> MAHHHHHHVGTDDWRCARSMHEFSAKDIDGHMVNLDKYRGFVCIVTNVASQCGKTEVNYTQL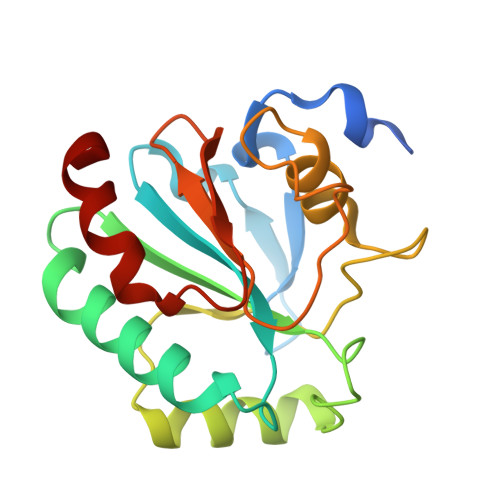VDLHARYAECGLRILLFPCNQFGKQEPGSNEEIKEFLAGYNFKGDAFSKICVNGDDAHPLWKWMKIQPKGKGILGNAIKWNFTKFLIDKNGCVVKRYGPMEEPLVIEKDLPHYF> VFPSSVYVPDEWEVSREKITLLRELGQGSFGMVYEGNARDIIKGEAETRVAVKTVNESASLRERIEFLNEASVMKGFTCHHVVRLLGVVSKGQPTLVVMELMAHGDLKSYLRSLRPEAENNPGRPPPTLQEMIQMAAEIADGMAYLNAKKFVHRDLAARNCMVAHDFTVKIGDFGMTRDIYETDYYRKGGKGLLPVRWMAPESLKDGVFTTSSDMWSFGVVLWEITSLAEQPYQGLSNEQVLKFVMDGGYLDQPDNCPERVTDLMRMCWQFNPNMRPTFLEIVNLLKDDLHPSFPEVSFFHSEENK;> SSQSISPMRSISENSLVAMDFSGQKSRVIENPTEALSVA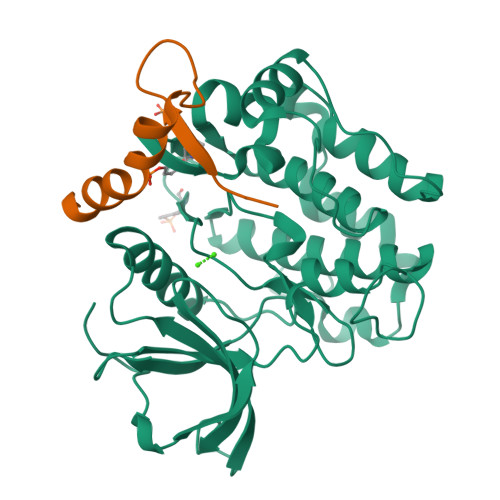VEEGLAWRKKGSLRLGTHGS> MKTQVAIIGAGPSGLLLGQLLHKAGIDNVILERQTPDYVLGRIRAGVLEQGMVDLLREAGVDRRMARDGLVHEGVEIAFAGQRRRIDLKRLSGGKTVTVYGQTEVTRDLMEAREACGATTVYQAAEVRLHDLQGERPYVTFERDGERLRLDCDYIAGCDGFHGISRQSIPAERLKVFERVYPFGWLGLLADTPPVSHELIYANHPRGFALCSQRSATRSRYYVQVPLSEKVEDWSDERFWTELKARLPSEVAEKLVTGPSLEKSIAPLRSFVVEPMQHGRLFLAGDAAHIVPPTGAKGLNLAASDVSTLYRLLLKAYREGRGELLERYSAICLRRIWKAERFSWW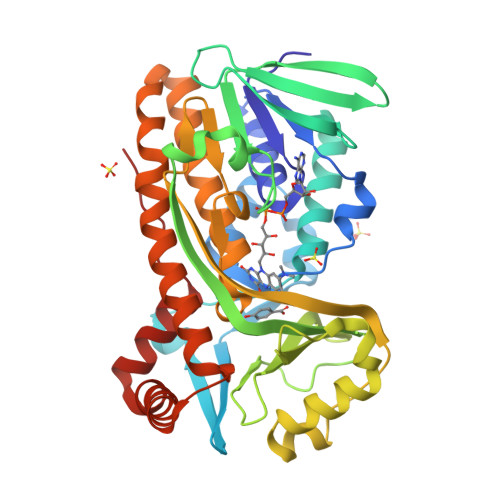MTSVLHRFPDTDAFSQRIQQTELEYYLGSEAGLATIAENYVGLPYEEIE>[8x]GSMPGFLTAFEYSEKRKMVFHITTGSQEFDKLLGGGIESMAITEAFGEFRTGKTQLSHTLCVTAQLPGAGGYPGGKIIFIDTENTFRPDRLRDIADRFNVDHDAVLDNVLYARAYTSEHQMELLDYVAAKFHEEAGIFKLLIIDSIMALFRVDFSGRGELAERQQKLAQMLSRLQKISEEYNVAVFVTNQMTADPGATMTFQADPKKPIGGHILAHASTTRISLRKGRGELRIAKIYDSPEMPENEATFAITAGGIGDAKE;>GRPTKVFVPPFKTK[7x]

BRCA2 is essential for DNA repair by homologous recombination in mitosis and meiosis. It interacts with recombinases RAD51 and DMC1 to facilitate the formation of nucleoprotein filaments on resected DNA ends that catalyse recombination-mediated repair. BRCA2’s BRC repeats bind and disrupt RAD51 and DMC1 filaments, whereas its PhePP motifs bind recombinases and stabilise their nucleoprotein filaments. Whilst Ex14 and Ex27 share an eponymous FxPP motif, their sequences are otherwise divergent, and they demonstrate specificity for DMC1- and RAD51-binding, respectively.

Hence, we established a crystallisation system for the structural core of human DMC1 in which its N-terminal domain was deleted (herein referred to as DMC1 ΔN; amino-acids 83–340). We then soaked DMC1 ΔN crystals with a peptide corresponding to a truncated form of BRCA2’s Ex14 (herein referred to as Ex14-Tr; amino-acids 2401-2414). Whilst soaking substantially reduced crystal quality, we obtained X-ray diffraction data to anisotropic resolution limits of 3.40–5.80 Å, in which additional peptide density was clearly observed. The electron density maps of the bound BRCA2 Ex14 peptide could not be interpreted unambiguously. Nevertheless, we were able to build the BRCA2 Ex14 structure guided by an AlphaFold2 model of the same BRCA2 Ex14 sequence bound to a DMC1 ΔN dimer. This resulted in a refined model of the peptide at seven out of the eight DMC1 protomers, with more extensive structural information at instances away from rather than at crystal lattice contacts. The observed BRCA2 Ex14 peptide contains the PhePP motif (amino-acids 2406-2409), in which F2406 is buried in a hydrophobic pocket and the two consecutive proline residues enable an unusual backbone conformation. The conformation of the Ex14 peptide was the same in all seven copies (r.m.s. deviation <0.4 Å), albeit with variation in the orientation of the F2410 side-chain and the C-terminus. The PhePP-binding site of DMC1 is formed by two loops, corresponding to amino-acids 147-153 and 178-183, respectively. DMC1’s PhePP-binding pocket includes V179 (L180 in RAD51) that mediates hydrophobic interactions with Ex14 amino acids P2409 and F2410.> YVLVPP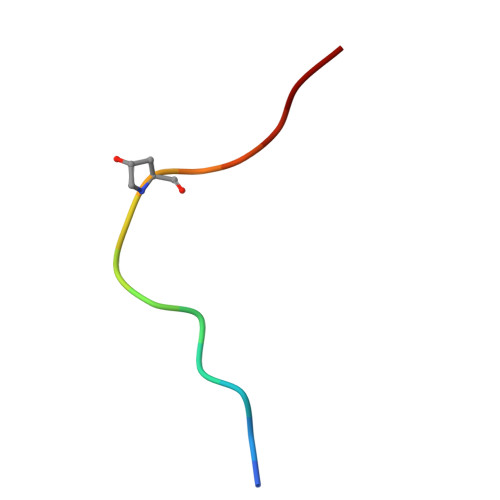SGPSMRHN> LFSQIELSFSASNLRDRDVLSKSDPMVVVYQKEKDATLSEVFRSEVVLNSLAPKWIKKFIVAYHFETVQTLVFRVYDVDTKFQNSREEMLKLDEQQFLGEATCALSEIITKSTRTSTLELKRKDGFAPQAQPHHGKLIIHAEESLASKISTEIVFRCSNLESKDLFSKSDPFLVVSKIVEHGTPIPVSKTEVRKNDLNPIWKPVFLSVQ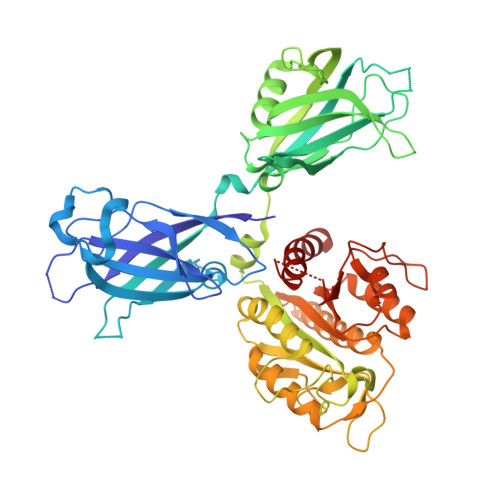QVGSKDSPVIIECSDFNSNGKHSLIGKVQKSLSDLEKLHLAGQGINFSLPTGAGQNKVLKSQLFVDKFTETVHHTFLEYLASGFELNFMVAIDFTASNGNPRLPDSLHYIDPSGRLNAYQRAIMDVGEVLQFYDSDKRFPAWGFGARPIDAPVSHCFNLNGSSSYSEVDGIQGIMTSYTSALFNVSLAGPTLFGPVINAAAMIASASLAQGSRKYYVLLIITDGVITDLQETKDALVSASDLPLSILIVGVGGADFKEMEILDADKGERLESSSGRLASRDIVQFVALRDVQYGEISVVQALLAELPSQFLTYMRIRN>QDKIKRVFVFGDSLT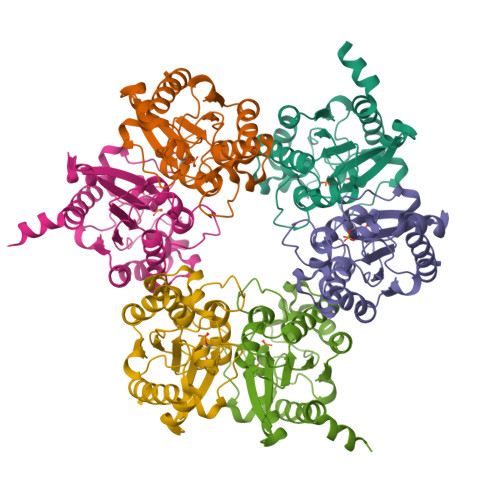WGWTPVAPIVPTTRHPHADRWTTVLGENLGDGYELVVDGLSGRTTNIDDPNDPKLNGADYLPAALAAHEPLDLVIILLGTNDTKTYLNRTPFEIGLGAGALINMVQKSPGWDWTDYPPPPVLLISPPPLGETIDPLAAPIFVDGLAKSEALPGVYKAIAEAAGESFFDAGSVVSTDGVDGIHFTAETNRTLGAAVAQKVKTLLQPKLAAALEHHHHHH[6x]> MHTAEFLETEPTEISSVLAGGYNHPLLRQWQSERQLTKNMLIFPLFISDNPDDFTEIDSAPNINRIGVNRLKDYLKPLVAKGLR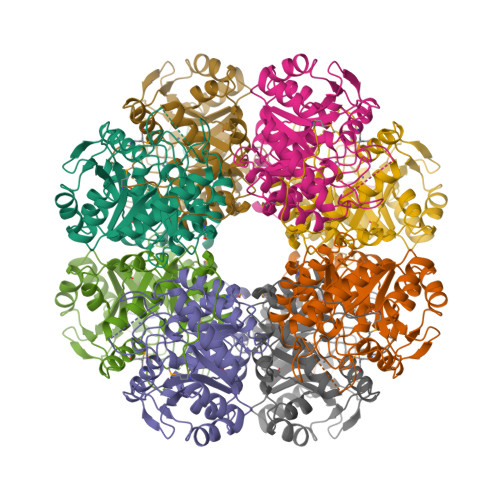SVILFGVPLIPGTKDPVGTAADDPAGPVIQGIRFIREKFPELYIICDVCLCEYTSHGHCGVLYDDGTINRERSVSRLAAVAVNYAKAGAHCVAPSDMIDGRIRDIKRGLINANLAHKTFVLSYAAKFSGNLYGPARDAACSAPSNGDRKCYQLPPAGRGLARRALERDMSEGADGIIVKPSTFYLDIVRDASEICKDLPICAYHVSGEYAMLHAAAEKGVVDLKTIAFESHQGFLRAGARLIITYLAPEFLDWLDE> GSHMKIKACIDEVTTTLEETKFLTNKLLLFADINGKLYHDSQNMLRGEDMSFLEKDAPYMVGDVITSGDITCVVIPSKKAGGTTEMLSRALKKVPVDEYITTYPGQGCAGYTLEEAKTALKKCKSAFYVLPSEAPNAKEEIL;> GSHMASMTGGQQMGRGSTLSEYVQDFLNHLTEQPGSFETEIEQFA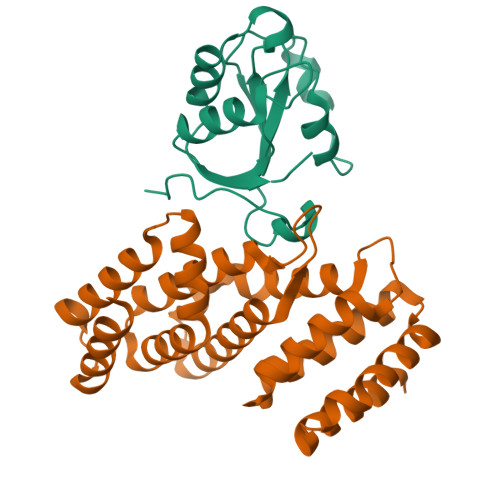ETLNGCVTTDDALQELVELIYQQATSIPNFSYMGARLCNYLSHHLTISPQSGNFRQLLLQRCRTEYEVKDQAAKGDEVTRKRFHAFVLFLGELYLNLEIKGTNGQVTRADILQVGLRELLNALFSNPMDDNLICAVKLLKLTGSVLEDAWKEKGKMDMEEIIQRIENVVLDANCSRDVKQMLLKLVELRSS> WSHPQFEKGAT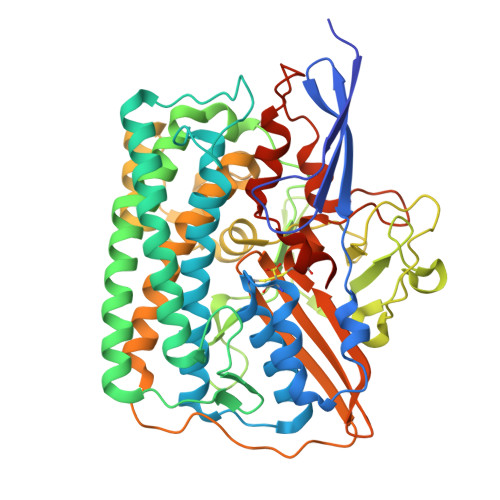GRTTIAIDPVTRIEGHLKAEVVVENGKVVDARLSGGMYRGFETILRGRDPRDASQIVQRICGVCPTAHSTASVLALDEAFGAKVPNNGRITRNLIFGANYLQSHILHFYHLSAQDFVQGPDTAPFVPRFPKSDLRLSKELNKAGVDQYIEALEVRRICHEMVALFGGRMPHVQGQVVGGATEIPTKEKLVEYAARFKKVRDFVEQKYVPVVYTIGSKYKDMFKVGQGFKAALCVGAFPLDNSGKKHLFMPGVYAKGKDMPFDPSKIKEYVKYSWFAEETTGLNYKEGKTIPAPDKAGAYSFVKAPRYDGLSLEVGPLARMWVNNPELSPVGKKLLKDLFGISAKKFRDLGEEAAFSLMGRHVARAEETYYMLGAIEGWLKEIKAGEDTVVMPAVPASAEGTGFTEAPRGSLLHYVKVKDSKIDNYQIVSASLWNCNPRDDMGQRGAVEEALIGIPVDDIQNPVNVARLIRAFDPULGCAVHVLHAESGKVAVIEVK(1R)-1-[((1E)-{3-HYDROXY-2-METHYL-5-[(PHOSPHONOOXY)METHYL]PYRIDIN-4-YL}METHYLENE)AMINO]-1-METHYLPROPYLPHOSPHONIC 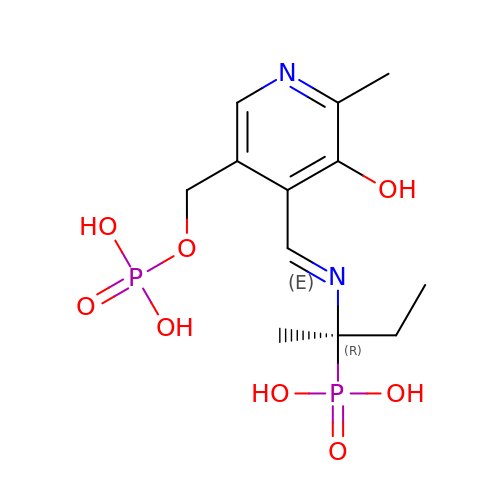ACID | C12 H20 N2 O8 P2 | CFHOMAMSGWRSCJ-CHJAJTDHSA-N> EQGNRPVETENIARGKQASQSSTAHGGAATRAVDGNVDSDYGHHSVTHTNFEDNAWWQVDLGKTENVGKVKLYNRGDGNVANRLSNFDVVLLNEAKQEVARQHFDSLNGKAELEVFFTAKDARYVKVELKTKNTPLSLAEVEVFRSATTQVGC

Lectinolysin (LLY) is a pore-forming toxin derived from some strains of Streptococcus mitis and S. pseudopneumoniae and is a member of the cholesterol-dependent cytolysin (CDC) family. While LLY shares a number of characteristics typical of CDCs, it has a unique 162 amino acid N-terminal domain (LLYlec; Farrand et al., 2008). Glycan array experiments revealed that LLY was highly selective for the difucosylated glycans Lewis y (Ley) and Lewis b (Leb) antigens. In the work presented here a Y62H mutation was designed and constructed with the aim of removing the hydrogen bond between the N-acetylglucosamine (GlcNAc) of Leb and LLYlec and instead, gain a hydrogen bond with Ley.

The structures of the LLYlecwt-Ley and LLYlecY62H-Ley superimpose very closely, with a rms deviation of the alpha carbon atoms of 0.1 Å. A third metal ion binding site is observed in the mutant structure and we have tentatively identified it as a Mg2+ ion binding site due to the very high concentrations of this ion in the crystallization buffer. The Mg2+ ion is bound between the carboxylate of Asp97 and the side-chain carbonyl of Gln54 and four water molecules, all arranged in octahedral geometry around the metal ion. The water structure is the same as in LLYlecwt-Ley apart from a water molecule that is positioned between the hydroxyl group of Tyr62 and fucose 1 (Fuc 1). This water molecule is shifted by 1.4 Å toward the NE2 of His62 in the mutant structure, compared to wild-type, to optimize its interaction with the His side-chain. LLYlecY62H forms the same 19 van der Waals interactions with Ley compared to the wild-type protein: 15 with Fuc 1, 1 with Gal, 2 with GlcNAc, and 1 with Fuc 2. The B-factor of Ley is 53.5 Å2 in the mutant (overall B-factor of protein is 29 Å2), compared to 38.2 Å2 in the wild-type protein (overall B-factor of protein complex is 21 Å2). Overall, there is no net change in the number of potential hydrogen binding and van der Waals interactions between wild-type and mutant Ley complexes. In the LLYlecY62H-Ley complex, there was no additional bond formation between the Lewis antigen and His62, only a shift of a water molecule toward the His, as compared to its position relative to Tyr62 in the wild-type. The mutation causes an overall 2.5-fold decrease in the lectin domain’s affinity for Ley and doubles its affinity for Leb over the wild-type domain.> MSQSNRELVVDFLSYKLSQKGYSWSQPMAAVKQALREAGDEFELRYRRAFSDLTSQLHITPGTAYQSFEQVVNELFRDGVNWGRIVAFF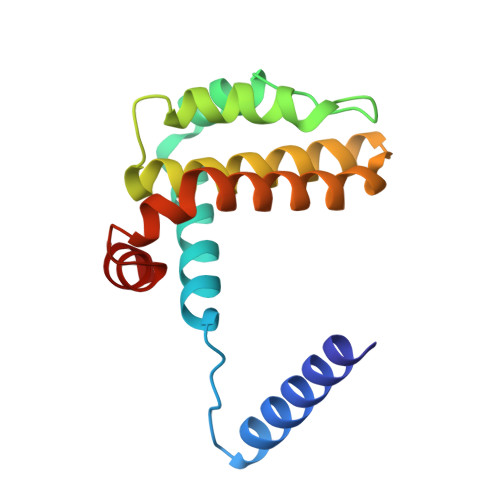SFGGALCVESVDKEMQVLVSRIASWMATYLNDHLEPWIQENGGWDTFVDLYG>CGCGAAUUC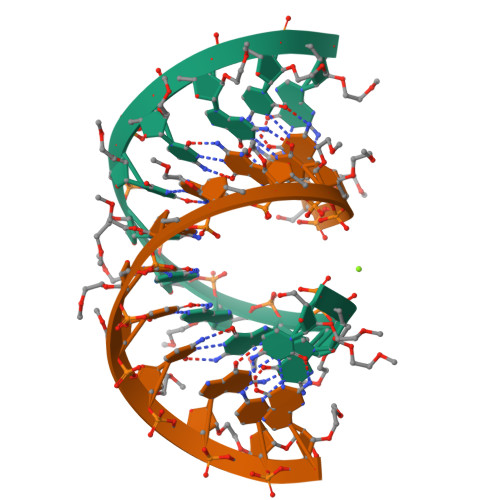GCG[2x]>[2x]MTMEKGMSSGEGLPSRSSQVSAGKITAKELETKQSYKEKRGGFVLVHAGAGYHSESKAKEYKHVCKRACQKAIEKLQAGALATDAVTAALVELEDSPFTNAGMGSNLNLLGEIECDASIMDGKSLNFGAVGALSGIKNPVSVANRLLCEGQKGKLSAGRIPPCFLVGEGAYRWAVDHGIPSCPPNIMTTRFSL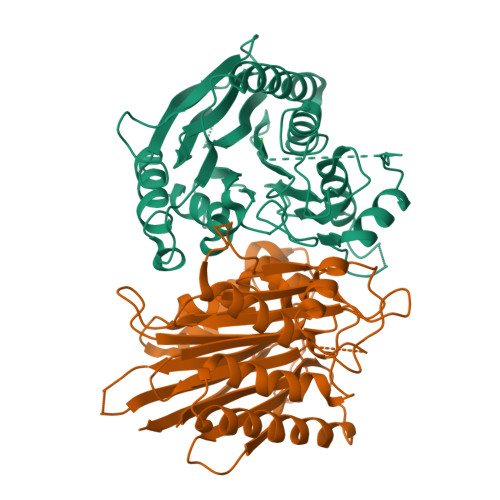AAFKRNKRKLELAERVDTDFMQLKKRRQSSEKENDSGTLDSVGAVVVDHEGNVAAAVSSGGLALKHPGRVGQAALYGCGCWAENTGAHNPYSTAVSTSGCGEHLVRTILARECSHALQAEDAHQALLETMQNKFISSPFLASEDGVLGGVIVLRSCRCSAEPDSSQNKQTLLVEFLWSHTTESMCVGYMSAQDGKAKTHISRLPPGAVAGQSVAIEGGVCRLESPVN>[6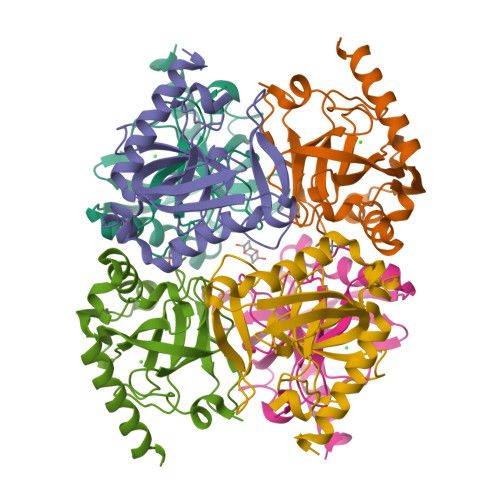x]MNPFHELEPGPEVPEVVYALIEIPKGSRNKYELDKKTGLLKLDRVLYSPFFYPVDYGIIPQTWYDDGDPFDIMVIMREPVYPLTIIEARPIGIMKMEDSGDKDWKVLAVPVEDPYFNDWKDISDVPKAFLDEIAHFFQRYKELQGKTTKIEGWGNAEEAKREILRAIEMYKEKFGKEE>MDKAKRNIKPFDGEKYAIWKFRIRALLAEQDVLKVVDGLMPNEVDDSWKKAERCAKSTIIEYLSDSFLNFATSDITARQILENLDAVYERKSLASQLALRKRLLSLKLSSEMSLLSHFHIFDELISELLAAGAKIEEMDKISHLLITLPSCYDGIITAIETLSE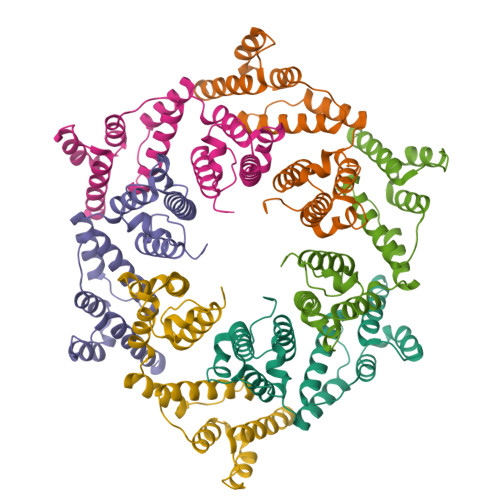ENLTLAFVKNRLLDQEIKIKNDHNDTSKKVMNAIVHNNNNTYKNNLFKNRVTKPKKIFKGNSKYKVKCHHCGREGHIKKDCFHYKRILNNKNKENEKQVQTATSHG[6x]> AERPTLPIPDLLTTDARNRIQLTIGAGQSTFGGKTATTWGYNGNLLGPAVKLQRGKAVTVDIYNQLTEETTLHWHGLEVPGEVDGGPQGIIPPGGKRSVTLNVDQPAATCWFHPHQHGKTGRQVAMGLAGLVVIEDDEILKLMLPKQWGIDDVPVIVQDKKFSADGQIDYQLDVMTAAVGWFGDTLLTNGAIYPQHAAPRGWLRLRLLNGCNARSLNFATSDNRPLYVIASDGGLLP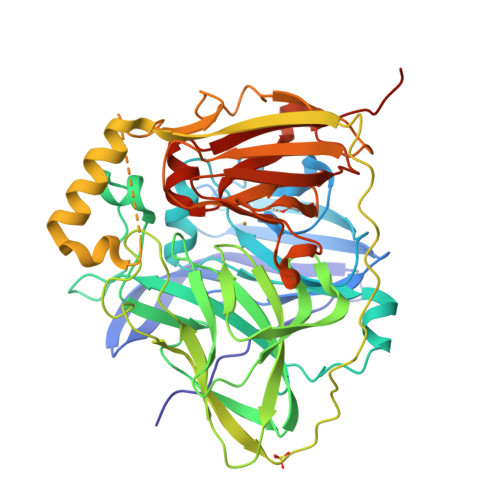EPVKVSELPVLMGERFEVLVEVNDNKPFDLVTLPVSQMGMAIAPFDKPHPVMRIQPIAISASGALPDTLSSLPALPSLEGLTVRKLQLSMDPMLDMMGMQMLMEKYGDQAMAGMDHSQMMGHMGHGNMNHMNHGGKFDFHHANKINGQAFDMNKPMFAAAKGQYERWVISGVGDMMLHPFHIHGTQFRILSENGKPPAAHRAGWKDTVKVEGNVSEVLVKFNHDAPKEHAYMAHSHLLEHEDTGMMLGFTVLQGDHGLSAWSHPQFEK> GSGAMERVLKVFHYFENSSEPTTWASIIRHGDATDVRGIIQKIVDCHKVKNVACYGLRLSHLQSEEVHWLHLDMGVSNVREKFELAHPPEEWKYELRIRYLPKGFLNQFTEDKPTLNFFYQQVKNDYMLEIADQVDQEIALKLGCLEIRRSYGEMRGNALEKKSNYEVLEKDVGLRRFFPKSLLDSVKAKTLRKLIQQTFRQFANLNREESILKFFEILSPVYRFDKECFKCALGSSWIISVELAIGPEEGISYLTDKGANPTHLADFNQVQTIQYSNSEDKDRKGMLQLKIAGAPEPLTVTAPSLTIAENMADLIDGYCRLVNGATQSFIIRPQKEGERALPSIPKLANNEKQGVRS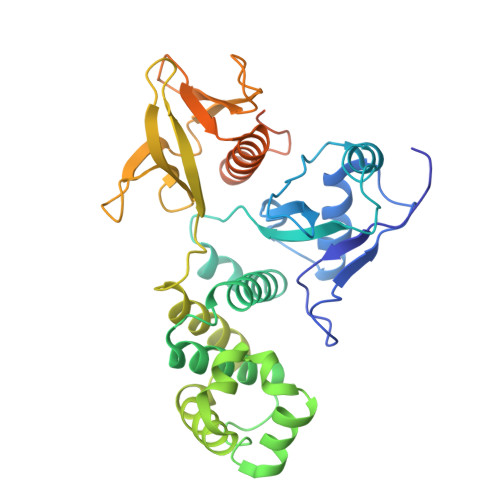HTVSVSETDDYAE>[12x]GSHMTTIGHLINGQLVTENTRSQNVFNPATGEIGKQLDLASTKTVEQAISAAQHAFPTWRNTPPLKRARVMFRFKELLEQHADEICRLIGEEHGKIAHDAMGELQRGIENVEYACGAPELLKGEHSRNVGPGIDSWSEFQPMGVVAGIT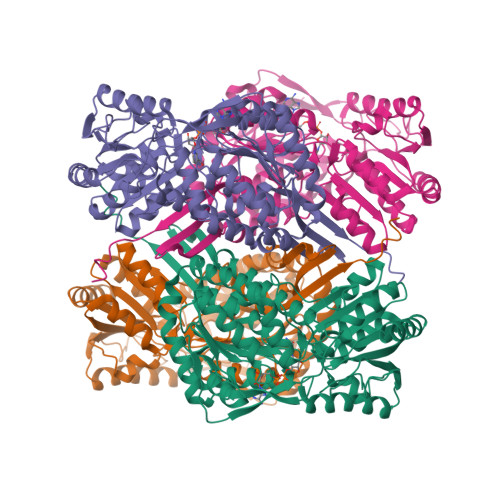PFNFPVMVPLWMFPMAIVCGNCFVLKPSERDPSSTLYIAQLLQEAGLPDGVMNVVNGDKEAVDALLHDDRVKAVSFVGSTPIAEYIYRTASANGKRCQALGGAKNHAIVMPDADMDNAVNQLLGAAFGSSGERCMALSVAVAVGDAAGDALVSKMTQAMQKLKVGPSTDSGNDFGPVITRQHQEKVIGYINSAEQQGATIVVDGRQPKVPNHENGFFVGGTLIDHVTPEMTSYQEEIFGPVLQVVRVATMQDAMDLIDAHEYGNGTCIFTRDGEAARYFSDNIQVGMVGINIPLPVPVAYHSFGGWKRSLFGDLHAYGPDAVRFYTKRKTVTQRWPSAGVREGAEFSMPTMK> GPDSMGAAAAEADRTLFVGNLETKVT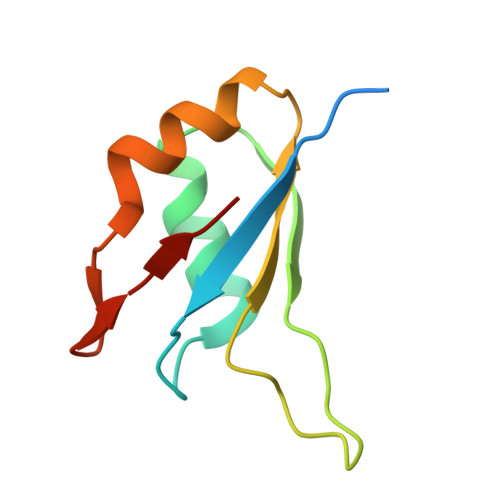EELLFELFHQAGPVIKVKIPKDKDGKPKQFAFVNFKHEVSVPYAMNLLNGIKLYGRPIKIQFRS> MRYLELAQLYQKLEKTTMKLIKTRLVADFLKKVPDDHLEFIPYLILGEVFPEWDERELGVGEKLLIKAVAMATGIDAKEIEESVKDTGDLGESIALAVKKKKQKSFFSQPLTIKRVYQTLVKVAETTGEGSQDKKVKYLADLFMDAEPLEAKYLARTILGTMRTGVAEGLLRDAIAMAFHVKVELVERAYMLTSDF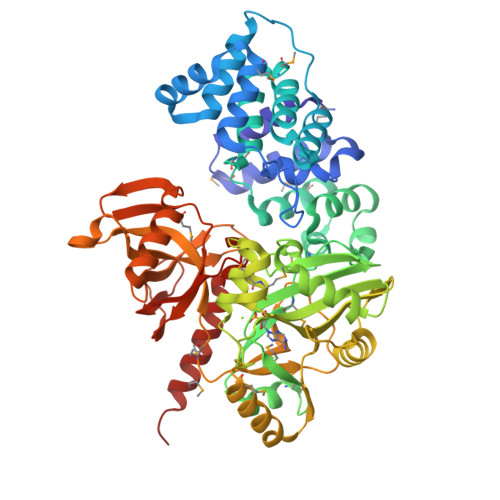GYVAKIAKLEGNEGLAKVQVQLGKPIKPMLAQQAASIRDALLEMGGEAEFEIKYDGARVQVHKDGSKIIVYSRRLENVTRAIPEIVEALKEAIIPEKAIVEGELVAIGENGRPLPFQYVLRRFRRKHNIEEMMEKIPLELNLFDVLYVDGQSLIDTKFIDRRRTLEEIIKQNEKIKVAENLITKKVEEAEAFYKRALEMGHEGLMAKRLDAVYEPGNRGKKWLKIKPTMENLDLVIIGAEWGEGRRAHLFGSFILGAYDPETGEFLEVGKVGSGFTDDDLVEFTKMLKPLIIKEEGKRVWLQPKVVIEVTYQEIQKSPKYRSGFALRFPRFVALRDDKGPEDADTIERIAQLYELQEKMKGKVES>[2x]SMPPKASKKDAAPAERPILGRFSSHLKIGIVGL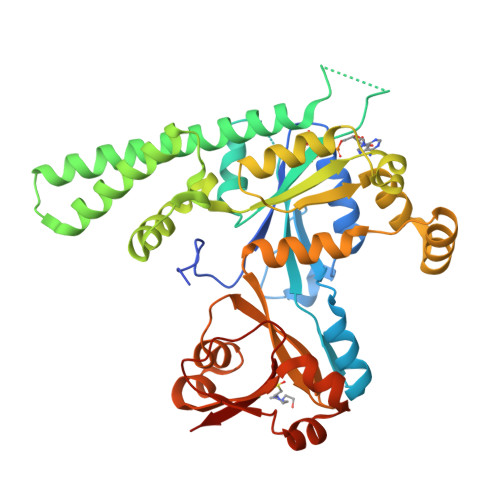PNVGKSTFFNIVTKLSIPAENFPFCTIDPNEARVYVPDERFDWLCQLYKPKSEVSAYLEINDIAGLVRGAHAGEGLGNAFLSHIRAVDGIFHVLRAFEDKEVTHIDDSVDPVRDLETIGEELRLKDIEFVQNKIDDLEKSMKRSNDKQLKLEHELCEKVKAHLEDGKDVRFGDWKSADIEILNTFQLLTAKPVVYLVNMSEKDYQRKKNKFLPKIHAWVQEHGGETIIPFSCAFERLLADMPPDEAAKYCAENQIASVIPKIIKTGFAAIHLIYFFTAGPDEVKCWQIRRQTKAPQAAGTIHTDFERGFICAEVMKFDDLKELGSESAVKAAGKYRQEGKTYVVQDGDIIFFKFNVSGGGKK> MAATAAEAVASGSGEPREEAGALGPAWDESQLRSYSFPTRPIPRLSQSDPRAEELIENEEPVVLTDTNLVYPALKWDLEYLQENIGNGDFSVYSASTHKFLYYDEKKMANFQNFKPRSNREE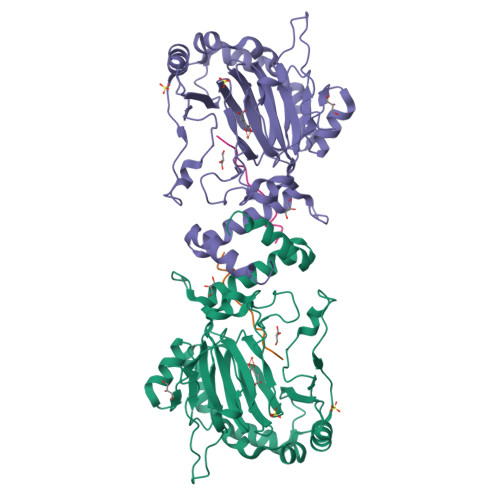MKFHEFVEKLQDIQQRGGEERLYLQQTLNDTVGRKIVMDFLGFNWNWINKQQGKRGWGQLTSNLLLIGMEGNVTPAHYDEQQNFFAQIKGYKRCILFPPDQFECLYPYPVHHPCDRQSQVDFDNPDYERFPNFQNVVGYETVVGPGDVLYIPMYWWHHIESLLNGGITITVNFWYKGAPTPKRIEYPLKAHQKVAIMRNIEKMLGEALGNPQEVGPLLNTMIKGRYN;> GMLEDLINSHADVNAVDD> MRRLAFLVVAFCLAVGCFFSPVSKAEGVMSGGDGDKVAVGKDGMVATAHPLASKIGAEVLKKGGNAIDAAIAIQYALNVTEPMMSGIGGGGFMMVYDGETKETSIINSRERAPEGAKPDMFLDEDGKVIPFSERSRHGNAVGVPGTLKGLEAAHKKWGTKKMEDLISPSIKLTEEGFPIDSVLADAIKDHQDKLSKTAAKDIFLPDGEPLKEGDILVQKDMAKTFKLIRKEGSKAFYDGEIGRAIADVVQDFGGSMTPDDLSRYEVTTDKPIWGEYHGYDIASMPPPSSGGVFMLQMLKLIDDFHLSQYDPKSFEKYHLLAETMHLSYADRAAYAGDPEFVDVPLRGLLDPDYIKERQKLISLDSMNRDVKEGDPWKYEEGEPNYEIVPQPEDKTIGE;> TTHFTVTDQWGNVVSYTTTIEQLFGTGILVPGYGLFLNNELTDFDAIPG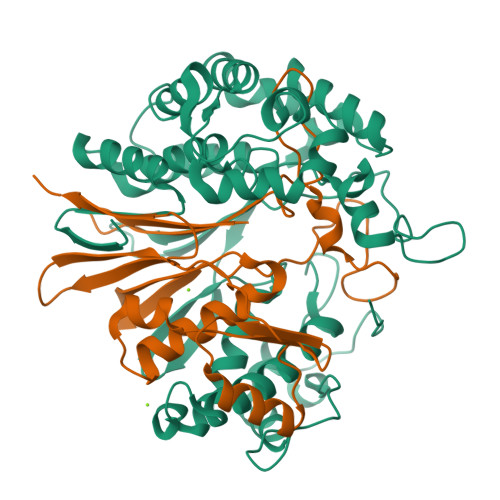GANEVQPNKRPLSSMTPTIVFKDEKPVLTVGSPGGTTIIASVFQTILNYFEYGMSLQDAIEEPRIYTNSLTSYRYESGMPEDVRRKLNDFGHKFGSNPVDIGNVQSIFIDRENKTFMGVADSSRNGTAVGVNIKTSAK WW domains organize molecular assemblies by binding to short, proline rich peptide motifs each with ~4–6 residues. The type I WW domains bind to a consensus ‘PPxY’ motif (where P is proline, x is any amino acid and Y is tyrosine, also known as PY-motif) with very modest affinities (with Kd in the range of a few to a few tens of µM). To achieve this goal, we determined the high resolustion structures of 7 representative WW tandem/target complexes, and measured the binding constants of >100 WW domain tandems or isolated WW domains binding to known or previously unknown targets. In this study, we discovered that WW tandems, but not individual WW domains, can bind to target proteins with extremely high affinity and with very high sequence specificity.

We found that the last canonical PY-motif of AMOT (the ‘PPEY’-motif, named as PY3 in the literature) is preceded with an ‘LMRY’-motif, and these two motifs are only separated with two residues (and we define these two motifs as ‘PY34’ from hereon). Unexpectedly, the KIBRA WW tandem binds to AMOT PY34 with a high affinity (Kd ~96 nM), although the PY3 sequence severely deviates from the canonical WW domain binding PY-motif of ‘PPxY’. We solved the high-resolution crystal structures of KIBRA WW tandems in complex with PTPN14 PY12, AMOT PY34 and LATS1 PY23. The interactions between WW2 and the first PY-motif are more variable, as their sequences can significantly deviate from the optimal ‘PPxY’-motif (e.g. AMOT’s 1st PY motif has an unusual ‘LMRY’ sequence). Correspondingly, KIBRA WW2 has an Ile (I81) instead of a highly conserved Trp at the end of the β3-strand (e.g. W34 in WW1). The Leu and Met in the PY3-motif of AMOT form hydrophobic interaction with I81 and Y70 from WW2. This explains why KIBRA WW2 can accommodate non-‘ΨPxY’ motif sequences, as long as the two residues corresponding to ‘Ψ’ and ‘P’ are hydrophobic. A residue in the PY-motif linker (R440 in PTPN14, Q282 in AMOT and G553 in LATS) uses its carbonyl group to form a hydrogen-bond with the sidechain of Trp34. The C-terminal extension of PTPN14 and that of AMOT form additional hydrophobic and charge-charge interactions with the WW1 domain. All these interactions contribute to the bindings of PTPN14 and AMOT to KIBRA WW tandem.

>[2x]GPGSEFELPLPEGWEEARDFDGKVYYIDHRNRTTSWIDPRDRYTKPLTFADCISDELPLGWEEAYDPQVGDYFIDHNTKTTQIEDPRVQWRREQEHMLKDYLVVAQEALSAQKEIYQVKQQRLELAQQEYQQLH;>[2x]GPGSGRTEGQLMRYQHPPEYGAARPA>[20x]MGSDKIHHHHHHMKIFLDTANLEEIKKGVEWGIVDGVTTNPT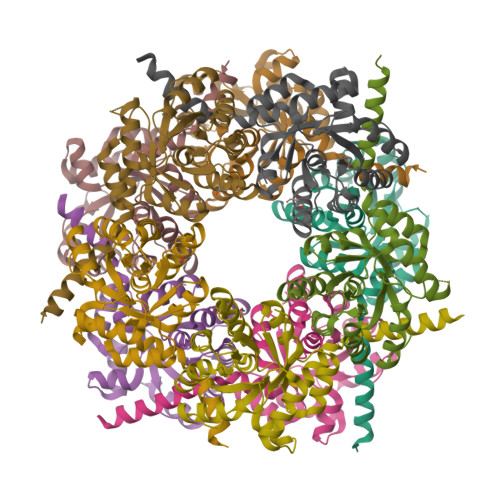LISKEGAEFKQRVKEICDLVKGPVSAEVVSLDYEGMVREARELAQISEYVVIKIPMTPDGIKAVKTLSAEGIKTNVTLVFSPAQAILAAKAGATYVSPFVGRMDDLSNDGMRMLGEIVEIYNNYGFETEIIAASIRHPMHVVEAALMGVDIVTMPFAVLEKLFKHPMTDLGIERFMEDWKKYLENLKK> MHHHHHHTSVMSHEFQLATAETWPNPWPMYRALRDHDPVHHVVPPQRPEYDYYVLSRHADVWSAARDHQTFSSAQGLTVNYGELEMIGLHDTPPMVMQDPPVHTEFRKLVSRGFTPRQVETVEPTVRKFVVERLEKLRANGGGDIVTELFKPLPSMVVAHYLGVPEEDWTQFDGWTQAIVAANAVDGATTGALDAVGSMMAYFTGLIERRRTEPADD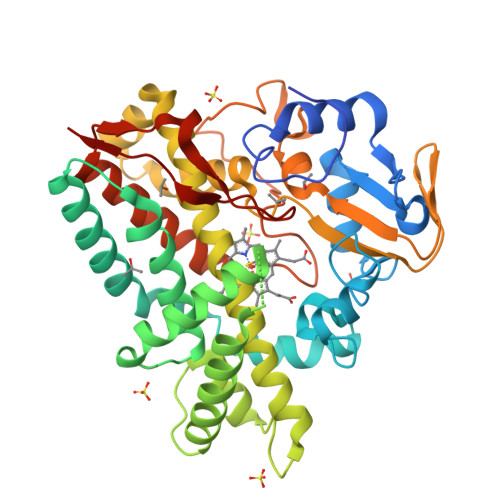AISHLVAAGVGADGDTAGTLSILAFTFTMVTAGNDTVTGMLGGSMPLLHRRPDQRRLLLDDPEGIPDAVEELLRLTSPVQGLARTTTRDVTIGDTTIPAGRRVLLLYGSANRDERQYGPDAAELDVTRCPRNILTFSHGAHHCLGAAAARMQCRVALTELLARCPDFEVAESRIVWSGGSYVRRPLSVPFRVTSSR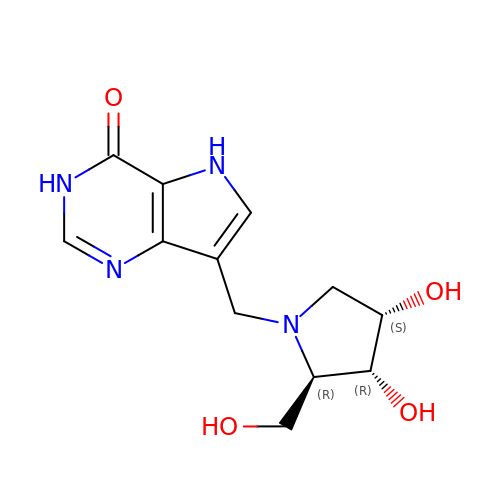7-(((2R,3R,4S)-3,4-dihydroxy-2-(hydroxymethyl)pyrrolidin-1-yl)methyl)-3H-pyrrolo[3,2-d]pyrimidin-4(5H)-one | C12 H16 N4 O4 | OKGGSJRJIFFOGK-VHSKPIJISA-N>SFAKGTNVLMADGSIECIENIEVGNKVMGKDGRPREVIKLPRGRETMYSVVQKSQHRAHKSDSSREVPELLKFTCNATNELVVRTPRSVRRLSRTIKGVEYFEVITFEMGQKKAPDGRIVELVKEVSKSYPISEGPERANELVESYRKASNKAYFEWTIEARDLSLLGSHVRKATYQTYAPILYENDHFFDYMQKSKFHLTIEGPKVLAYLLGLWIGDGLSDRATFSVDSRDTSLMERVTEYAEKLNLCAEYKDRKEPQVAKTVNLYSKVVRGNGIRNNLNTENPLWDAIVGLGFLKDGVKNIPSFLSTDNIGTRETFLAGLIDSDGYVTDEHGIKATIKTIHTSVRDGLVSLARSLGLVVSVNAEPAKVDMNGTKHKISYAIYMSGGDVLLNVLSKCAGSKKFRPAPAAAFARECRGFYFELQELKEDDYY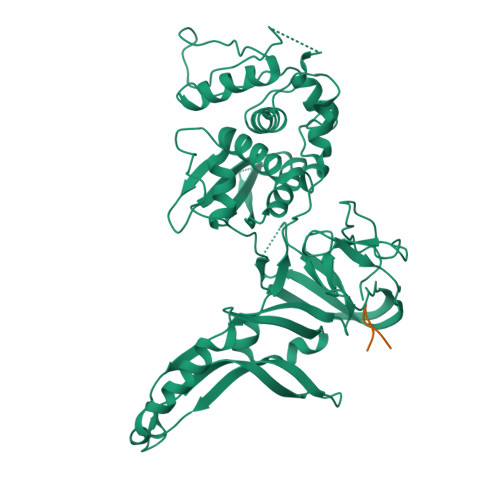GITLSDDSDHQFLLANQVVVHN[2x];>MSNSDAIIYVGSGERGNEMAE[2x]>MEETVDPNQKVIALTFSDGPNPATTNQILDSLKKYKGHATFFVLGSRVQYYPETLIRMLKEGNEVGNHSWSHPLLTRLSVKEALKQINDTQDIIEKISGYRPTLVRPPYGGINDELRSQMKMDVALWDVDPEDWKDRNKKTIVDRVMNQAGDGRTILIHDIYRTSADAADEIIKKLTDQGYQLVTVSQLEEVKKQREAKELRRQWSHP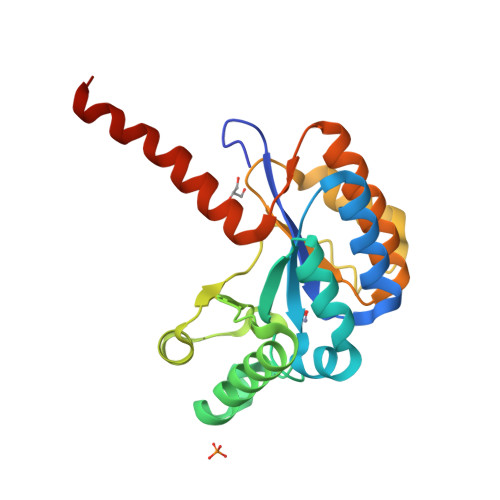QFEK[2x]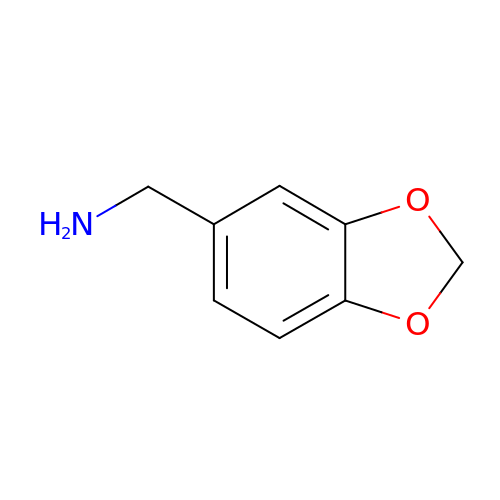1-(1,3-BENZODIOXOL-5-YL)METHANAMINE | C8 H9 N O2 | ZILSBZLQGRBMOR-UHFFFAOYSA-N3-amino-D-alanine | C3 H8 N2 O2 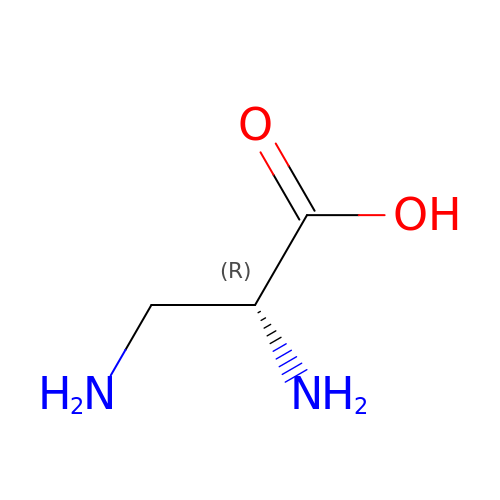| PECYZEOJVXMISF-UWTATZPHSA-N> APNGKKKNWKKIMTMSTKYKWTRTKIDIAEGPGSMNMANVLCTTGAQSVALVGERAFYDPRTAGSKSRFDDLVKIAQLFSVMADSTTPSENHGVDAKGYFKWSATTAPQSIVHRNIVYLRLFPNLNVFVNSYSYFRGSLVLRLSVYASTFNRGRLRMGFFPNATTDSTSTLDNAIYTICDIGSDNSFEITIPYSFST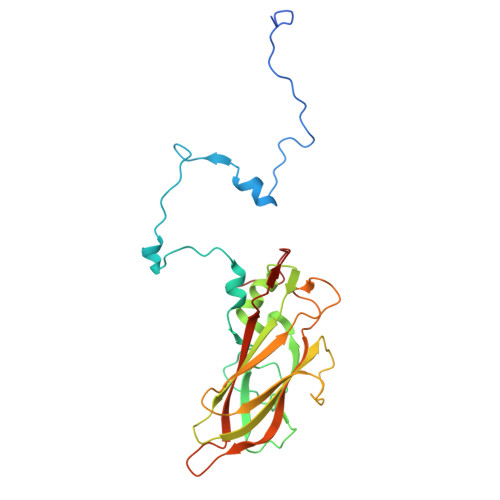WMRKTNGHPIGLFQIEVLNRLTYNSSSPSEVYCIVQGKMGQDARFFCPTGSVVTFQ> MSSTNIEQVMPVKLAQALANPLFPALDSALRSGRHIGLDELDNHAFLMDFQE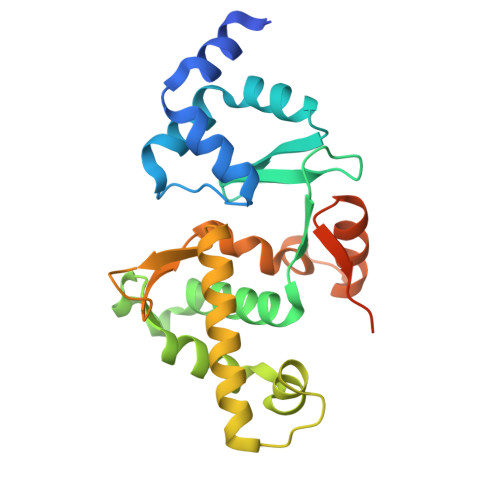YLEEFYARYNVELIRAPEGFFYLRPRSTTLIPRSVLSELDMMVGKILCYLYLSPERLANEGIFTQQELYDELLTLADEAKLLKLVNNRSTGSDVDRQKLQEKVRSSLNRLRRLGMVWFMGHDSSKFRITESVFRFGADVRAGDDPREAQRRLIRDGEAMPIENHLQLNDETEENQPDSGEEE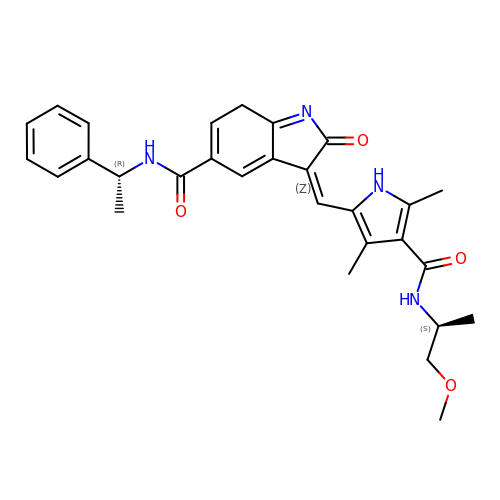(3Z)-3-[(4-{[(2S)-1-methoxypropan-2-yl]carbamoyl}-3,5-dimethyl-1H-pyrrol-2-yl)methylidene]-2-oxo-N-[(1R)-1-phenylethyl]-3,7-dihydro-2H-indole-5-carboxamide | C29 H32 N4 O4 | JDMXFAOBJOWKMQ-NVULIICISA-N>SNAAPAPAPAPEVQTKHFTLKSDVLFNFNKSTLKPEGQQALDQLYSQLSNLDPKDGSVVVLGFTDRIGSDAYNQGLSEKRAQSVVDYLISKGIPSDKISARGMGESNPVTGNTCDNVKPR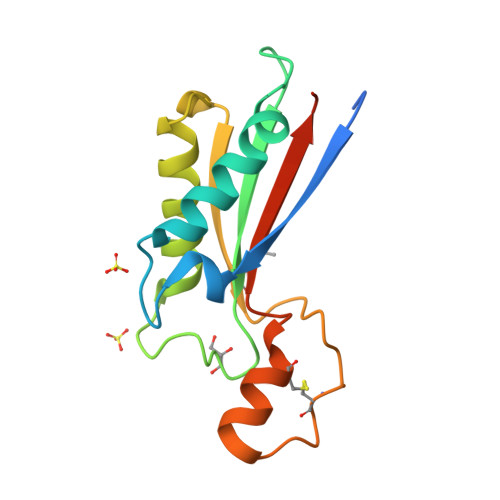AALIDCLAPDRRVEIEVKGVKDVVTQPQ[2x]> DTVGRPLPHLAAAMQASGEAVYCDDIPRYENELFLRLVTSTRAHAKIKSIDVSEAQKVPGFVCFLSADDIPGSNETGLFNDETVFAKDTVTCVGHIIGAVVADTPEHAERAAHVVKVTYEDLPAIITIEDAIKNNSFYGSELKIEKGDLKKGFSEADNVVSGELYIGGQDHFYLETHCTIAIPKGEEGEMELFVSTQNAMKTQSFVAKMLGVPVNRILVRVKRMGGGFGGKETRSTLVSVAVALAAYKTGHPVRCMLDRNEDMLITGGRHPFLARYKVGFMKTGTIVALEVDHYSNAGNSRDLSH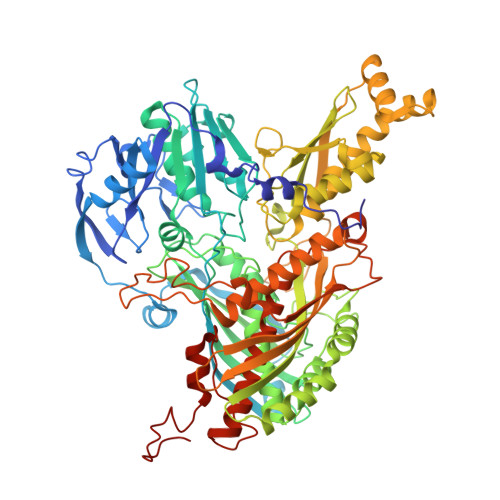SIMERALFHMDNCYKIPNIRGTGRLCKTNLSSNTAFRGFGGPQALFIAENWMSEVAVTCGLPAEEVRWKNMYKEGDLTHFNQRLEGFSVPRCWDECLKSSQYYARKSEVDKFNKENCWKKRGLCIIPTKFGISFTVPFLNQAGALIHVYTDGSVLVSHGGTEMGQGLHTKMVQVASKALKIPISKIYISETSTNTVPNSSPTAASVSTDIYGQAVYEACQTILKRLEPFKKKNPDGSWEDWVMAAYQDRVSLSTTGFYRTPNLGYSFETNSGNAFHYFTYGVACSEVEIDCLTGDHKNLRTDIVMDVGSSLNPAIDIGQVEGAFVQGLGLFTLEELHYSPEGSLHTRGPSTYKIPAFGSIPTEFRVSLLRDCPNKKAIYASKAVGEPPLFLGASVFFAIKDAIRAARAQHTNNNTKELFRLDSPATPEKIRNACVDKFTTLCVTGAPGNCKPWSLRV>[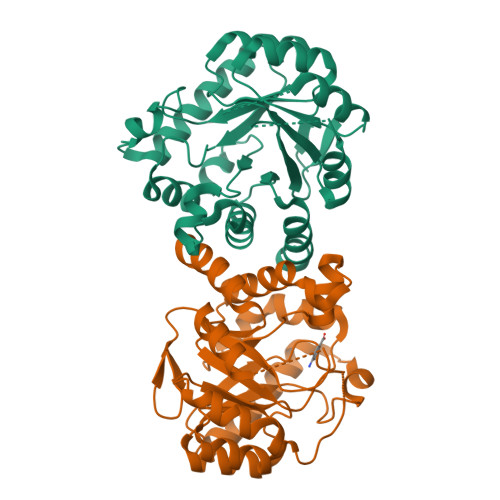2x]MGAPPLGPTIIPPVRTLWLRDRALDLDRVRLLGVLNLTPDSFSDGGRYLDPERALERAREMVAEGADILDLGAESTRPGAAPVPVEEEKRRLLPVLEAVLSLGVPVSVDTRKPEVAEEALKLGAHLLNDVTGLRDERMVALAARHGVAAVVMHMPVPDPATMMAHARYRDVVAEVKAFLEAQARRALSAGVPQVVLDPGFGFGKLLEHNLALLRRLDEIVALGHPVLVGLSRKRTIGELSGVEDPAQRVHGSVAAHLFAVMKGVRLLRVHDVRAHREALGVWEALYGGDRPSRA>[2x]MLKKRGYDVTRNPHLNKGMAFTLEERLQLGIHGLIPPCFLSQDVQLLRIMRYYERQQSDLDKYIILMTLQDRNEKLFYRVLTSDVEKFMPIVYTPTVGLACQHYGLTFRRPRGLFITIHDKGHLATMLNSWPEDNIKAVVVTDGERILGLGDLGCYGMGIPVGKLALYTACGGVNPQQCLPVLLDVGTNNEELLRDPLYIGLKHQRVHGKAYDDLLDEFMQAVTDKFGINCLIQFEDFANANAFRLLNKYRNKYCMFNDDIQGTASVAVAGILAALRITKNKLSNHVFVFQGAGEAAMGIAHLLVMALEKEGVPKAEATRKIWMVDSKGLIVKGRSHLNHEKEMFAQDHPEVNSLEEVVRLVKPTAIIGVAAIAGAFTEQILR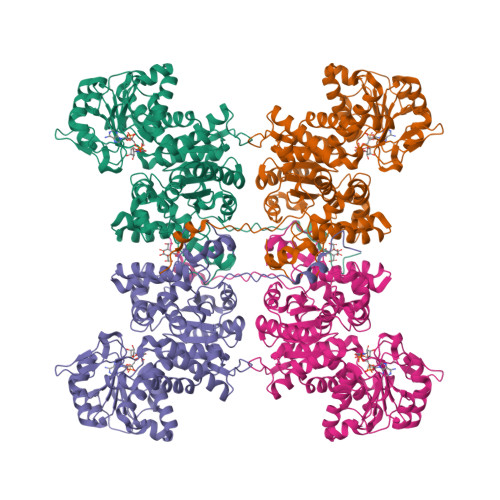DMASFHERPIIFALSNPTSKAECTAEKCYRVTEGRGIFASGSPFKSVTLEDGKTFIPGQGNNAYVFPGVALGVIAGGIRHIPDEIFLLTAEQIAQEVSEQHLSQGRLYPPLSTIRDVSLRIAIKVLDYAYKHNLASYYPEPKDKEAFVRSLVYTPDYDSFTLDSYTWPKEAMNVQTVTRENLYFQ>[3x]SM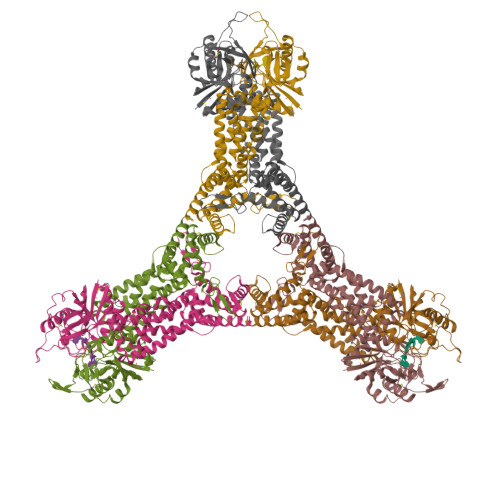KCLFYIAGDVSNYSIVNYELNGQTQNTFFAAHALYNLFKPDKVIALIPDSLVKDNVSDEECYKNLVINRAKELNFAGMEEFMNKVEIRKIPNVGIASAIQCENGAPKKEKNKEGREVLKRLPYNEKRSPIFIFNAIYAIFKDEACDEYLVDLTHGTNVLVSIGMNVGALFNAKFYSAPVMGMPGKDSIVNIVELTDVVQATNDSLMIRSSIENLDERYFKDYSAKLSRLNPTIFEEEEKKVLTRVKGTDVNVVINFLWNIRNGFTVNAVKSMNELKNIINQLEEDLEKLKSFYKNWEEHKNFQGETLLVLSDLDSTLKVKDLLIEGNDLEKLNYLLDLYIKASIYDKALSLARELPVAICLNKVGGGMFDDKNEKYKHCNEIVTSYLRLRYSGLMEFRNTLMHGGLSTDMKPNVDKDGNITPGKIVTKNKIEDFVKRELRNYFDKIVNFLSSA Scribble is a highly conserved regulator of cell polarity, a process that enables the generation of asymmetry at the cellular and tissue level in higher organisms. Scrib belongs to the LAP (leucine-rich repeats and PDZ domain) protein family, and features sixteen LLRs (Leucine-rich repeats), two LAP-specific domains (LAPSDa and LAPSDb) and the four PDZ domains (PDZ1, PDZ2, PDZ3 and PDZ4). The influenza A virus NS1 protein was shown to bind to human Scribble (SCRIB) via its C-terminal PDZ binding motif (PBM). Examination of the SCRIB PDZ:NS1 complexes showed that the NS1 peptides are bound in the canonical ligand-binding groove formed by the β2 strand and helix α2.

We determined crystal structures of SCRIB PDZ1 bound to NS1 ESEV PBM (A281-R219-T220-I221-E222-S223-E224-V225), SCRIB PDZ1 bound to NS1 ESKV PBM (A281-R219-T220-I221-E222-S223-K224-V225) and PDZ3 bound to NS1 ESKV PBM (A281-R219-T220-I221-E222-S223-K224-V225). In the SCRIB PDZ3:ESKV complex, Val225ESKV is docked in the conserved hydrophobic pocket formed by SCRIB PDZ3 Leu1014, Gly1014 and Leu1016. Additionally, hydrogen bonds are formed between Lys224ESKV-Leu1016SCRIB PDZ3, Ser223ESKV-Ile1018SCRIB PDZ3 and Ser223ESKV-His1071SCRIB PDZ3 at the α2 helix. Glu222ESKV side-chain reaches over to the β2 strand and forms an ionic bond with the Lys1039SCRIB PDZ2. Although SCRIB PDZ3 K1040 formed an ionic bond with ESKV seen in the SCRIB PDZ3:ESKV complex, it appears not to be a critical contributor to the overall affinity, with loss of the interaction only modestly reducing the overall affinity of the SCRIB PDZ3:PBM interaction. SCRIB PDZ3 K1040A showed a weaker interaction with ESEV (22.2 ± 1.1 µM) and ESKV (13.8 ± 0.8 µM) compared to the wild-type SCRIB PDZ3 counterpart (ESEV:13.1 ± 1.6 µM, ESKV:12.1 ± 0.9 µM). SCRIB PDZ3 H1071A revealed complete loss of binding for both ESEV and ESKV, whereas PDZ3 K1040A interacted with both (ESEV: 22.2 ± 1.1 µM) (ESKV: 13.8 ± 0.8 µM). Our ITC analysis of the ESKV PBM revealed an interaction with SCRIB PDZ2 (KD = 9.5 ± 0.7 µM) as the tightest interactor, followed by SCRIB PDZ3 (KD = 12.1 ± 0.9 µM) and SCRIB PDZ1 (KD = 30.0 ± 0.9 µM) as the weakest interactor. Interestingly, there were no significant differences in the interaction of SCRIB PDZ3 (β-PIX:14.7 ± 2.1 µM, ESEV: 13.1 ± 1.6 µM, ESKV:12.1 ± 0.9 µM). Additionally, S1026PDZ3 interacts with the β-PIX W641, whereas S1026PDZ3 is not involved in the SCRIB PDZ3:ESKV complex; instead, a K1040PDZ3-E222ESKV hydrogen bond is formed.

>[4x]GGSVEEIRLPRAGGPLGLSIVGGSDHSSHPFGVQEPGVFISKVLPRGLAARSGLRVGDRILAVNGQDVRDATHQEAVSALLRPCLELSLLVRRD;>[4x]KMARTIESKV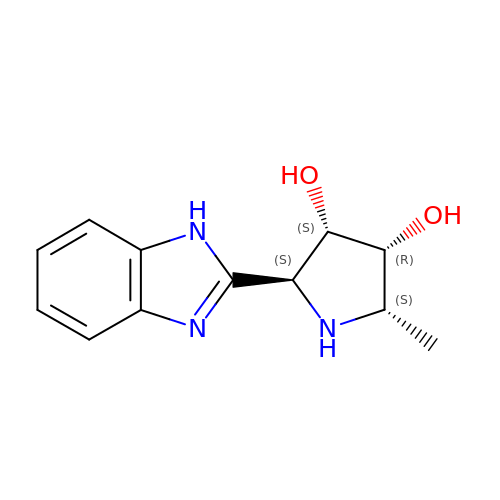(2S,3S,4R,5S)-2-(1H-benzimidazol-2-yl)-5-methylpyrrolidine-3,4-diol | C12 H15 N3 O2 | WKDUAKZZRFRSAE-HCPDIIQCSA-N> KVFERCELARTLKRLGMDGYRGISLANWMCLAKWESGYNTRATNYNAG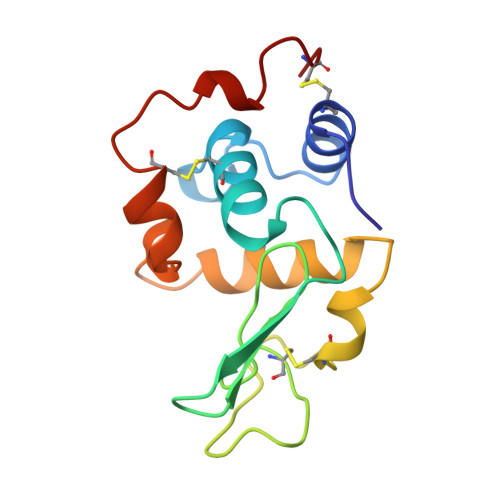DRSTDYGIFQINSRYWCNDGKTPGAVNAAHLSCSALLQDNIADAVAAAKRVARDPQGIRAWVAWRNRCQNRDVRQYVQGCGV> MGSNQSSSTSTKKLKAGNFDVAYQNPDKAIKGGNLKVAYQSDSPMKAQWLSGLSNDATFATMSGPGGGQDGLFFTDSGFKFIKGGAADVALDKESKTATITLRKDLKWSDGSEVTAKDYEFTYETIANPAYGSDRWTDSLANIVGLSDYHTGKAK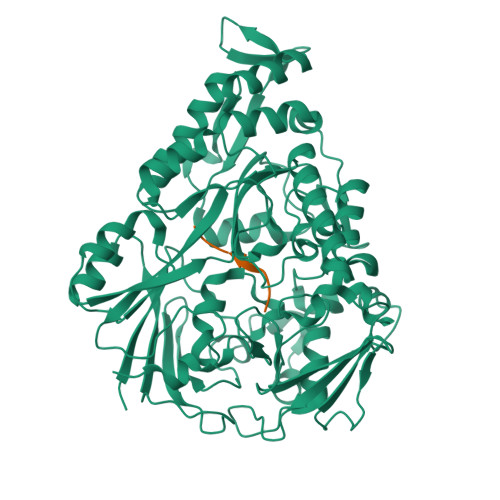TISGITFPDGENGKVIKVQFKEMKPGMTQSGNGYFLETVAPYQYLKDVAPKDLASSPKTTTKPLVTGPFKPENVVAGESIKYVPNPYYWGEKPKLNSITYEVVSTAKSVAALSSSKYDIINGMVSSQYKQVKNLKGYKVLGQQAMYISLMYYNLGHYDAKNSINVQDRKTPLQDQNVRQAIGYARNVAEVDNKFSNGLSTPANSLIPPIFKQFTSSSVKGYEKQDLDKANKLLDEDGWKLNKSTGYREKDGKELSLVYAARVGDANAETIAQNYIQQWKKIGVKVSLYNGKLMEFNSWVDHMTTPPGANDWDITDGSWSLASEPSQQDLFSAAAPYNFGHFNDSEITKDLNDIDSAKSENPTYRKAAFVKYQEDMNKKAYVIPTNFMLNYTPVNKRVVGMTLDYGAMNTWSEIGVSSAKLATKGSIEGRHHHHHH;> ASNSIASG> CPAR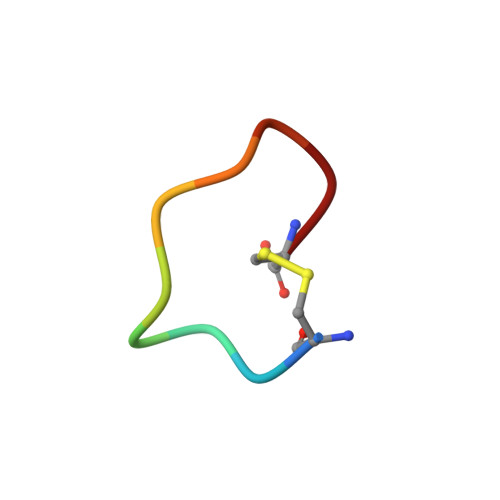FAALFC>MSDKDSKNTPQVPEKLGLSRRGFLGASAVTGAAVAATALGGAVMTRESWAQAVKESKQKIHVGPGELDDYYGFWSGGHQGEVRVLGVPSMRELMRIPVFNVDSATGWGLTNESRHIMGDSAKFLNGDCHHPHISMTDGKYDGKYLFINDKANSRVARIRLDIMKCDKMITVPNVQAIHGLRLQKVPHTKYVFANAEFIIPHPNDGKVFDLQDENSYTMYNAIDAETMEMAFQVIVDGNLDNTDADYTGRFAAATCYNSEKAFDLGGMMRNERDWVVVFDIHAVEAAVKAGDFITLGDSKTPVLDGRKKDGKDSKFTRYVPVPKNPHGCNTSSDGKYFIAAGKLSPTCSMIAIDKLPDLFAGKLADPRDVIVGEPELGLGPLHTTFDGRGNAYTTLFIDSQVVKWNMEEAVRAYKGEKVNYIKQKLDVHYQPGALHASLCETNEADGKWLVALSKFSKDRFLPVGPLHPENDQLIDISGDEMKLVHDGPTFAEPHDCIMARRDQIKTKKIWDRNDPFFAPTVEMAKKDGINLDTDNKVIRDGNKVRVYMTSMAPAFGVQEFT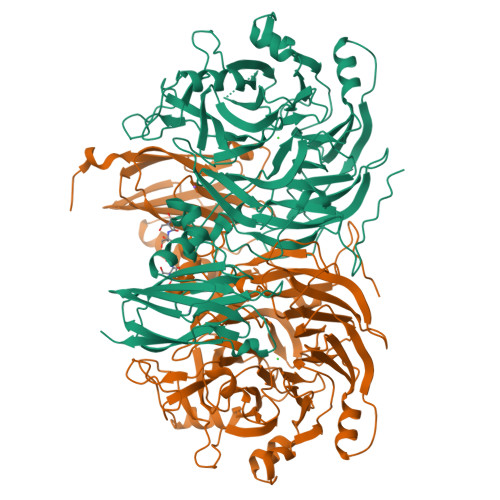VKQGDEVTVTITNIDQIEDVSHGFVVVNHGVSMEISPQQTSSITFVADKPGLHWYYCSWFCHALHMEMVGRMMVEPAWSHPQFEK[2x]>[3x]MN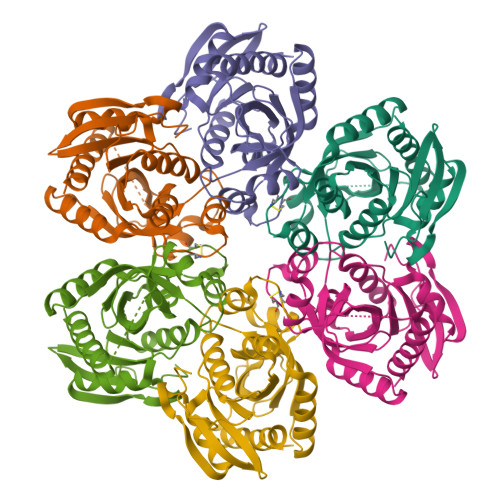PVHILAKKGEVAERVLVVGDPGRARLLSTLLQNPKLTNENRGFLVYTGKYNGETVSIATHGIGGPSIAIVLEELAMLGANVFIRYGTTGALVPYINLGEYIIVTGASYNQGGLFYQYLRDNACVASTPDFELTNKLVTSFSKRNLKYYVGNVFSSDAFYAEDEEFVKKWSSRGNIAVEMECATLFTLSKVKGWKSATVLVVSDNLAKGGIWITKEELEKSVMDGAKAVLDTLTS> GSMMLSLNNLQNIIYNPVIPFVGTIPDQLDPGTLIVIRGHVPSDADRFQVDLQNGSSVKPRADVAFHFNPRFKRAGCIVCNTLINEKWGREEITYDTPFKREKSFEIVIMVLKDKFQVAVNGKHTLLYGHRIGPEKIDTLGIYGKVNIHSIGFSFSSHMRLPFAARLNTPMGPGRTVVVKGEVNANAKSFNVDLLAGKSKDIALHLNPRL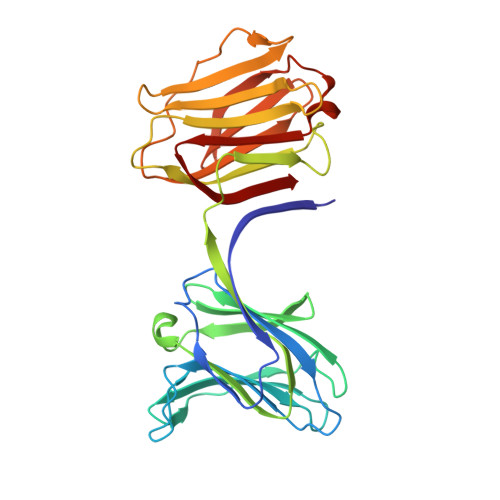NIKAFVRNSFLQESWGEEERNITSFPFSPGMYFEMIIYCDVREFKVAVNGVHSLEYKHRFKELSSIDTLEINGDIHLLEVRSW>[2x]GSDELYRQSLEIISRYLREQATGAKDTKPMGRSGATSRKALETLRRVGDGVQRNHETAFQGMLRKLDIKNEDDVKSLSRVMIHVFSDGVTNWGRIVTLISFGAFVAKHLKTINQESCIEPLAESITDVLVRTKRDWLVKQRGWDGFVEFFHVEDLE;>[2x]XQWVREIAAGLRRAADDVNAQVERX

Anti-apoptotic members of the Bcl-2 family are broadly recognized as promising cancer therapeutic targets. Human anti-apoptotic proteins Bcl-2, Bcl-xL, Bcl-w, Mcl-1 and Bfl-1 have a globular, helical fold and function by binding to short, α-helical Bcl-2 homology 3 (BH3) motifs in pro-apoptotic proteins, as shown in Figure 1A. Competition for binding among BH3-containing proteins regulates mitochondrial outer membrane permeabilization (MOMP), which is an irreversible step toward caspase activation and cell death. The role of anti-apoptotic protein Bfl-1 in cancer is less characterized than that of Mcl-1 or Bcl-xL, but many lines of evidence suggest that Bfl-1 is also a critical target. Thus, Bfl-1 is an intriguing therapeutic target and biomarker for resistance to cytotoxic anticancer drugs.

Crystals of the Mcl-1/FS2 peptide complex were grown at room temperature in hanging drops over a reservoir containing 0.2 M zinc sulfate, 0.1 M imidazole (pH 6.5), and 3% 6-aminohexanoic acid. The protein was mixed with peptide at a 1:1 molar ratio and diluted to 2 mg/ml in 20 mM Tris, 150 mM NaCl, 1% glycerol, 1 mM DTT, pH 8.0. Crystals were cryoprotected by transferring into 15% glycerol, 0.2 M zinc sulfate, 0.1 M imidazole (pH 6.5) and 3% 6-aminohexanoic acid prior to flash freezing. For example, the structures of FS2 bound to Bfl-1 can be used to design chemical crosslinks to reinforce helicity and promote cellular uptake, the structure of FS2 bound to Mcl-1 can be used to further reduce Mcl-1 binding, and the structure of FS2_1fX can be used as a platform for the design of therapeutic peptides and small molecules that covalently target Bfl-1.>MFENITATTADPILGLADLFRADERPGKIDLGIGVYKDETGKTPVLTSVKKAE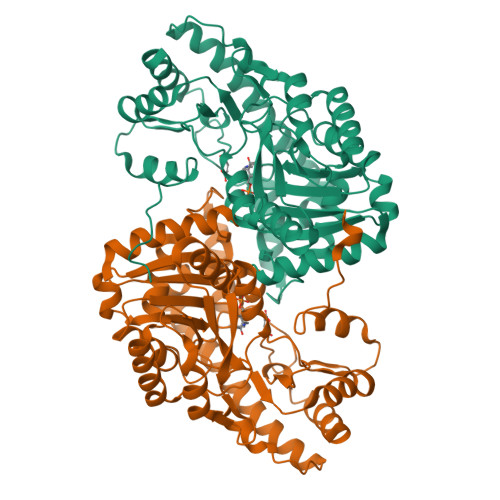QYLLENETTKNYLGIDGIPEFGRCTQELLFGKGSALINDKRARTAQTPGGSGALRVAADFLAKNTSVKRVWVSNPSWPNHKSVFNSAGLEVREYAYYDAENHTLDFDALINSLNEAQAGDVVLFHGCCHNPTGIDPTLEQWQTLAQLSVEKGWLPLFDFAYQGFARGLEEDAEGLRAFAAMHKELIVASSYSKNFALYNERVGACTLVAADSETVDRAFGQMKAAIRANYSSPPAHGASVVATILSNDALRAIWEQELTDMRQRIQRMRQLFVNTLQEKGANRDFSFIIKQNGMFSFSGLTKEQVLRLREEFGVYAVASGRVNVAGMTPDNMAPLCEAIVAVL[2x]>MSLNARARALRHSRSGTIGLIVPDVNNAVFADMFSGVQMAASGHSTDVLLGQIDAPPRGTQQLSRLVSEGRVDGVLLQRREDFDDDMLAAVLEGVPAVTINSRVPGRVGSVILDDQKGGGIATEHLITLGHSRIAFISGTAIHDTAQRRKEGYLETLASAGLRSEAAWVVDAGWEADAGSAALNTLYRGANLGKPDGPTAVVVASVNAAVGALSTALRLGLRVPEDLSIVGINTTWVSDTVYPALTTVRLPLQRLGEVAADVLMEHLGGRALTDTVVTQPTPELLVR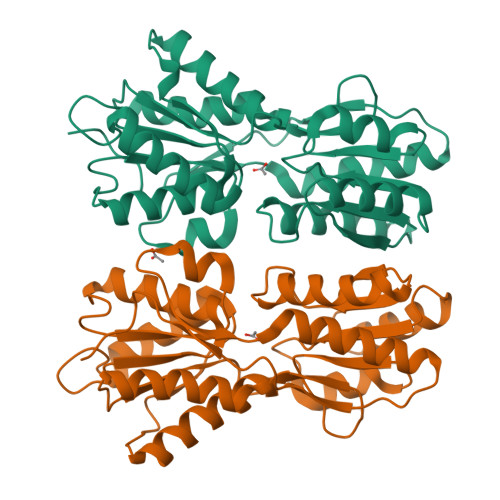ETTAPPTREGHHHHHH[4x]> GSHMMPGEIRPTIGQQMETGDQRFGDLVFRQLAPNVWQHTSYLDMPGFGAVASNGLIVRDGGRVLVVDTAWTDDQTAQILNWIKQEINLPVALAVVTHAHQDKMGGMDALHAAGIATYANALSNQLAPQEGMVAAQHSLTFAANGWVE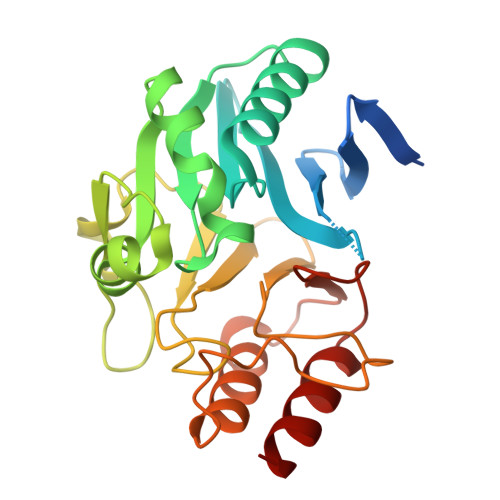PATAPNFGPLKVFYPGPGHTSDNITVGIDGTDIAFGGCLIKDSKAKSLGNLGDADTEHYAASARAFGAAFPKASMIVMSHSAPDSRAAITHTARMADKLR Strigolactones (SLs) and karrikins (KARs) are two classes of structurally related molecules that mediate signaling pathways to stimulate seed germination. SL and KAR have been reported to be recognized by the homologous proteins D14 (DWARF14)14–17 and HTL (HYPOSENSITIVE TO LIGHT; also known as KAI2, KARRIKIN INSENSITIVE2), respectively. To elucidate the structural basis of ligand specificity, we determined the crystal structures of ShHTL1, ShHTL4, ShHTL7, and ShD14 and compared their structures with those reported for ShHTL331 and ShHTL529. All the structures were highly similar to one another, consisting of a canonical α/β hydrolase domain and a helical cap.

Y150 was changed to F150 in a subgroup (ShHTL4, ShHTL5, and ShHTL7) of the divergent clade, thus losing the hydrogen bond between helices αD1 and αD3. Therefore, helices αD1 and αD2 of ShHTL4, ShHTL5, and ShHTL7 slid away from αD3, resulting in larger pockets with a reduced chance of causing steric hindrance with ligands. This finding is interesting because ShHTL4, ShHTL5, and ShHTL7 have been shown to be highly sensitive to various natural SLs (polyspecific receptors) in a previous study. In the divergent clade (ShHTL4, ShHTL5, and ShHTL7), ShHTL7 had the largest pocket. For example, ShHTL7, with the largest pocket, had the helix αD1 tilting the greatest extent away from the entrance of the pocket. Structural analyses revealed that although the cap domains of ShHTL7 could overlay well with those of ShHTL4 and ShHTL5, with a root-mean-square deviation (RMSD) of 0.9 Å, ShHTL7 had more non-bulky residues than ShHTL4 and ShHTL5, such as T142, L153, and T157. It is reasoned that ShHTL7 evolved to use smaller residues to enlarge its pocket while sustaining activity. To verify the importance of pocket size for ligand recognition of ShHTLs, a double mutation T190F/C194F and a triple mutation L124F/T190F/C194F of ShHTL7 were generated to introduce large side-chain amino acids to reduce the pocket size by partially mimicking ShHTL3. The inhibition constant Kirac-GR24 in the YLG competition assays was used to indicate the rac-GR24 binding affinity of ShHTL7. It is shown that the T190F/C194F mutation led to a twofold decrease, and the L124F/T190F/C194F mutation led to more than a 100-fold decrease in the rac-GR24 binding affinity. Our results showed that rac-GR24 triggered the interaction of ShHTL7 with ShMAX2, which was consistent with the results of a previous study.

>[4x]MGMSSIGLAHNVTILGSGETTVVLGHGYGTDQSVWKLLVPYLVDDYKVLLYDHMGAGTTNPDYFDFDRYSSLEGYSYDLIAILEEFQVSKCIYVGHSMSSMAAAVASIFRPDLFHKLVMISPTPRLINTEEYYGGFEQKVMDETLRSLDENFKSLSLGTAPLLLACDLESAAMQEYCRTLFNMRPDIACCITRMICGLDLRPYLGHVTVPCHIIQSSNDIMVPVAVGEYLRKNLGGPSVVEVMPTEGHLPHLSMPEVTIPVVLRHIRQDITDHTRHHHHHH> MAMSEALEIIDFGDSKARTDTEHLAINNETGYRSFRAGGFTFTRDEYFARLTWPGGSHIIPIDAFLRAMMRDVAWGFFYGVVNFDHVFGTINHYGEVTMFAGRFNDAYRNAGRDHEERFKSSALMAVFKDILSDWTVEGYDPFAAPMETGLPWGIKNGNNDEAISRQRVTARRMVGLPGDTPVRTDANGFPVNRQFADVPQEQPVVEAEPGFEAEVSAYNLFGYLSRSDVTWNPSVCSVVGDSLFCPTSEEFILPVEHGNDRCEWFLQLSD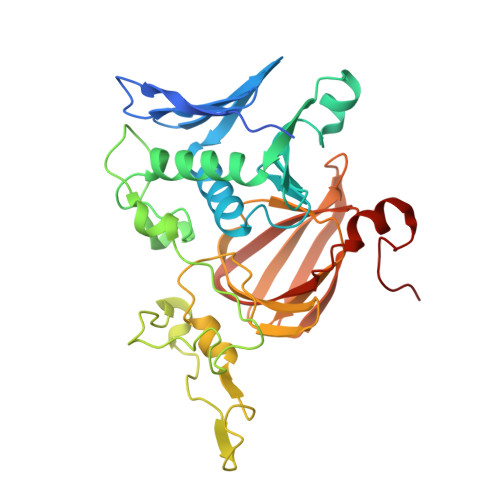EIVWDVKDKESGKPRARVTARAGDICCMPADIRHQGYSTKRSMLLVWENGSPKIPQMIADGTAPVVPVTF>MENTENSVDSKSIKNLEPKIIHGSESMDSGISLDNSYKMDYPEMGLCIIINNKNFHKSTGMTSRSGTDVDAANLRETFRNLKYEVRNKNDLTREEIVELMR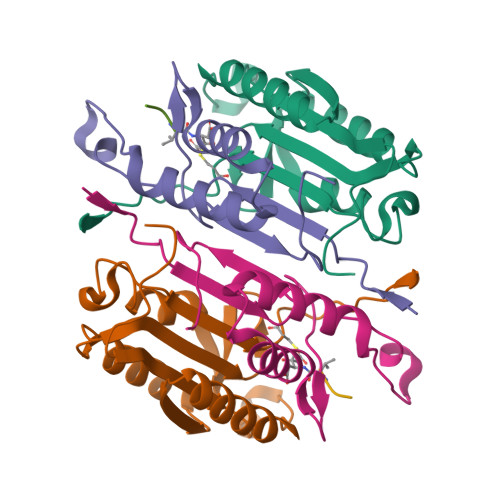DVSKEDHSKRSSFVCVLLSHGEEGIIFGTNGPVDLKKITNFFRGDRCRSLTGKPKLFIIQACRGTELDCGIETD[2x];>[2x]SGVDDDMACHKIPVEADFLYAYSTAPGYYSWRNSKDGSWFIQSLCAMLKQYADKLEFMHILTRVNRKVATEFESFSFDATFHAKKQIPCIVSMLTKELYFYHLEHHHHHH3-[6-{2'-[(DIMETHYLAMINO)METHYL]BIPHENYL-4-YL}-7-OXO-3-(TRIFLUOROMETHYL)-4,5,6,7-TETRAHYDRO-1H-PYRAZOLO[3,4-C]PYRIDIN-1-YL]BENZAMIDE 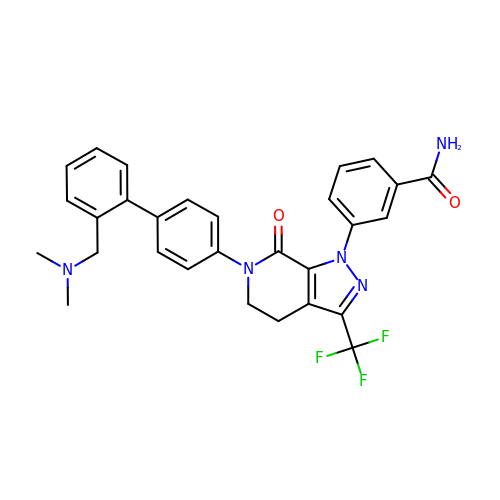| C29 H26 F3 N5 O2 | PKGPGSWPKRHPKB-UHFFFAOYSA-N>MTGSNSHITILTLNINGLNSAIKRHRLASWIKSQDPSVCCIQETHLTCRDTHRLKIKGWRKIYQANGKQKKAGVAILVSDKTDFKPTKIKRDKEGHYIMVKGSIQQEELTILNIYAPNTGAPRFIKQV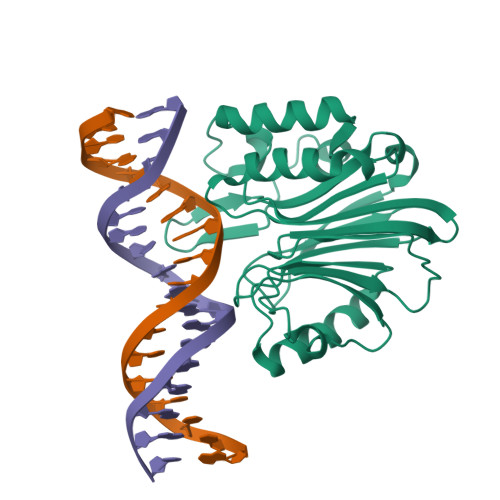LSDLQRDLDSHTLIMGAFNTPLSTLDRSTRQKVNKDTQELNSALHQADLIDIYRTLHPKSTEYTFFSAPHHTYSKIDHIVGSKALLSKCKRTEIITNKLSDHSAIKLELR[2x]>AECS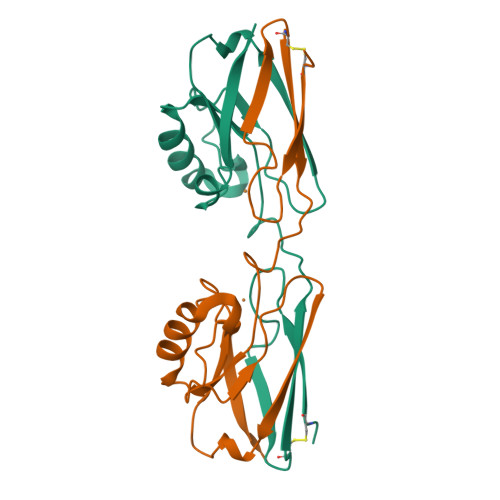VDIAGNDQMQFDKKEITVSKSCKQFTVNLKHPGKLAKNVMGHNWVLTKQADMQGAVNDGMAAGLDNNYVKKDDARVIAHTKVIGGGETDSVTFDVSKLAAGQDYAYFCSFPGHFALMKGVLKLVD[4x]>MYSTAVLLNKISPTRDGQTMTLADLQYLSFSELRKIFDDQLSWGEARHLYHETIEQKKNNRLLEARIFTRANPQLSGAIRLGIERDSVSRSYDEMFGARSSSFVKPGSVASMFSPAGYLTELYREAKDLHFSSSAYHLDNRRPDLADLTLSQSNMDTEISTLTLSNELLLEHITRKTGGDSDALMESLSTYRQAIDTPYHQPYETIRQVIMTHDSTLSALSRNPEVMGQAEGASLLAILANISPELYNILTEEITEKNADALFAQNFSENITPENFASQSWIAKYYGLELSEVQKYLGMLQNGYSDSTSAYVDNISTGLVVNNESKLEAYKITRVKTDDYDKNINYFDLMYEGNNQFFIRANFKVSREFGATLRKNAGPSGIVGSLSGPLIANTNFKSNYLSNISDSEYKNGVKIYAYRYTSSTSATNQGGGIFTFESYPLTIFALKLNKAIRLCLTSGLSPNELQTIVRSDNAQGIINDSVLTKVFYTLFYSHRYALSFDDAQVLNGSVINQYADDDSVSHFNRLFNTPPLKGKIFEADGNTVSIDPDEEQSTFARSALMRGLGVNSGELYQLGKLAGVLDAQNTITLSVFVISSLYRLTLLARVHQLTVNELCMLYGLSPFNGKTTASLSSGELPRLVIWLYQVTQWLTEAEITTEAIWLLCTPEFSGNISPEISNLLNNLRPSISEDMAQSHNRELQAEILAPFIAATLHLASPDMARYILLWTDNLRPGGLDIAGFMTLVLKESLNANETTQLVQFCHVMAQLSLSVQTLRLSEAELSVLVISGFAVLGAKNQPAGQHNIDTLFSLYRFHQWINGLGNPGSDTLDMLRQQTLTADRLASVMGLDISMVTQAMVSAGVNQLQCWQDINTVLQWIDVASALHTMPSVIRTLVNIRYVTALNKAESNLPSWDEWQTLAENMEAGLSTQQAQTLADYTAERLSSVLCNWFLANIQPEGVSLHSRDDLYSYFLIDNQVSSAIKTTRLAEAIAGIQLYINRALNRIEPNARADVSTRQFFTDWTVNNRYSTWGGVSRLVYYPENYIDPTQRIGQTRMMDELLENISQSKLSRDTVEDAFKTYLTRFETVADLKVVSAYHDNVNSNTGLTWFVGQTRENLPEYYWRNVDISRMQAGELAANAWKEWTKIDTAVNPYKDAIRPVIFRERLHLIWVEKEEVAKNGTDPVETYDRFTLKLAFLRHDGSWSAPWSYDITTQVEAVTDKKPDTERLALAASGFQGEDTLLVFVYKTGKSYSDFGGSNKNVAGMTIYGDGSFKKMENTALSRYSQLKNTFDIIHTQGNDLVRKASYRFAQDFEVPASLNMGSAIGDDSLTVMENGNIPQITSKYSSDNLAITLHNAAFTVRYDGSGNVIRNKQISAMKLTGVDGKSQYGNAFIIANTVKHYGGYSDLGGPITVYNKTKNYIASVQGHLMNADYTRRLILTPVENNYYARLFEFPFSPNTILNTVFTVGSNKTSDFKKCSYAVDGNNSQGFQIFSSYQSSGWLDIDTGINNTDIKITVMAGSKTHTFTASDHIASLPANSFDAMPYTFKPLEIDASSLAFTNNIAPLDIVFETKAKDGRVLGKIKQTLSVKRVNYNPEDILFLRETHSGAQYMQLGVYRIRLNTLLASQLVSRANTGIDTILTMETQRLPEPPLGEGFFANFVLPKYDPAEHGDERWFKIHIGNVGGNTGRQPYYSGMLSDTSETSMTLFVPYAEGYYMHEGVRLGVGYQKITYDNTWESAFFYFDETKQQFVLINDADHDSGMTQQGIVKNIKKYKGFLNVSIATGYSAPMDFNSASALYYWELFYYTPMMCFQRLLQEKQFDEATQWINYVYNPAGYIVNGEIAPWIWNCRPLEETTSWNANPLDAIDPDAVAQNDPMHYKIATFMRLLDQLILRGDMAYRELTRDALNEAKMWYVRTLELLGDEPEDYGSQQWAAPSLSGAASQTVQAAYQQDLTMLGRGGVSKNLRTANSLVGLFLPEYNPALTDYWQTLRLRLFNLRHNLSIDGQPLSLAIYAEPTDPKALLTSMVQASQGGSAVLPGTLSLYRFPVMLERTRNLVAQLTQFGTSLLSMAEHDDADELTTLLLQQGMELATQSIRIQQRTVDEVDADIAVLAESRRSAQNRLEKYQQLYDEDINHGEQRAMSLLDAAAGQSLAGQVLSIAEGVADLVPNVFGLACGGSRWGAALRASASVMSLSATASQYSADKISRSEAYRRRRQEWEIQRDNADGEVKQMDAQLESLKIRREAAQMQVEYQETQQAHTQAQLELLQRKFTNKALYSWMRGKLSAIYYQFFDLTQSFCLMAQEALRRELTDNGVTFIRGGAWNGTTAGLMAGETLLLNLAEMEKVWLERDERALEVTRTVSLAQFYQALSSDNFNLTEKLTQFLREGKGNVGASGNELKLSNRQIEASVRLSDLKIFSDYPESLGNTRQLKQVSVTLPALVGPYEDIRAVLNYGGSIVMPRGCSAIALSHGVNDSGQFMLDFNDSRYLPFEGISVNDSGSLTLSFPDATDRQKALLESLSDIILHIRYTIRS[5x]

ABC toxin complexes (Tcs) are a class of α-pore forming toxins (αPFTs) that consist of three subunits capable of assembling into a single protein apparatus with the ability to shuttle and translocate toxic peptides into target cells. The two TcAs termed Xn-XptA1 and Xn-XptA2 are the targeting components of each complex and display variations in insect specificity. The TcAs are the largest subunits of the complex and contain a translocation channel with hydrophobic loops at the end allowing for membrane permeation. Upon TcA binding and an environmental pH change, the complex undergoes a conformational change into an active state in which the translocation channel is exposed and pierces the target cell membrane.

We separated particle subsets based on structural variations in 2D and 3D classifications indicative of RBD A mobility and observed the State 2 intermediate in the Xn-XptA2 wt data. We were able to resolve the Xn-XptA2 wt State 2 structure to 3.9 Å resolution, leading us to conclude that the State 2 structure is a physiological intermediate state preceding the pore state conformational change in Xn-XptA2 wt. Upon closer inspection of the region around RBD A in both Xn-XptA2 State 2 structures, we observed an opening in the outer shell of the protein where RBD A pivots outward. The narrowest area of this pore in the Xn-XptA2 wt State 2 structure has a maximum radius of 4.28 Å that is surrounded by four amino acids from two separate protomers: D518 (Chain A), Q152 (Chain E), D156 (Chain E), and S291 (Chain A). Comparatively, in the Xn-XptA2 YWKT structure, the narrowest constriction point in the pore has a maximum radius of 4.6 Å and is also compressed by four amino acids from two separate protomers: D518 (Chain A), Q152 (Chain E), Q294 (Chain A), and K291 (Chain A). This pore leads into the inner cavity space between the outer shell and the outside of the α-pore forming domains that make up the translocation channel. The NDs are located at the tip of the TcA and based on our current understanding of membrane perforation of TcAs, would most likely encounter cell surface receptors or the membrane of the target cell. This makes it reasonable to conclude that once Xn-XptA2 contacts cell surface receptors or the cell membrane, this mechanical stress stimulates Xn-XptA2 to undergo a conformational change from the canonical pre-pore state or State 1 to the newly discovered alternative State 2. From this, we propose that once Xn-XptA2 encounters a target receptor, the protein undergoes a conformational change from State 1 to State 2 to allow an influx of solvent, presumably in the insect midgut at very basic pH levels, into the inner cavity to further stimulate an additional conformational change leading into the pore state transition.>MGGEIITLQAGQCGNHVGKFLWSQLAKEHAIGTDGLSQLPDSSTERDDDTKPFFRENSRNKFTPRAIMMDSEPSVIADVENTFRGFFDPRNTWVASDGASAGNSWANGYDIGTRNQDDILNKIDKEIDSTDNFEGFQLLHSVAGGTGSGLGSNLLEALCDRYPKKILTTYSVFPARSSEVVVQSYNTILALRRLIEDSDATVVFDNASLLNISGKVFRNPNIDLQHTNQLISTIISSVTNSIRFPSYMYSSMSSIYSTLIPSPELHFLSPSFTPFTSDYIHDDIAHKGHSSYDVMLDLLDPSNSLVSTAMNNPTYFNVYNTIIGNVEPRQISRAMTKLQQRIKFPSWSSSAMHVNIGRRSPYLPLQPNENEVSGMMLSNMSTVVNVFENACNTFDKVFAKGAFLNNYNVGDLFQSMQNVQDEFAESREVVQSLMEDYVAAEQDSYLDDVLVDDENMVGELEEDLDADGDHKLV[2x];> MEIKEVDDRAELLRYTNNIPLLGKLVNHQPLWSTNPKLKSFSLEKISAPDQRRVQEALVVKDLLNVLIGLEGTYIRYFNDYEPSDPETPIEFKIAKKMDPSFKTFSRRIVRYGKQYMILTRAYEKWSDTSFGMVLQRFAYEIRRFLEDVYLKTLVERLERDFNKVPNFSIRELEQIINETEVNKQMELLYNIYEEIFREIEERRTNQSSQEDFNNFMDSMKNESSLHLRLMVAFDTTVYPVPKGGAILKIFQQKILENLGDRSSVMFLKKLLNNISQDYCTMLYEWLTQGILNDPYQEFMTYDDLEGKTDNIFDTRDRAWDTQYFIRKDVLLRDCDSEEDKNLLFKMLRTGILLKVVRASLQIPTIPSNSSDITIQEINDFADLMEGSNLELYVDKCYSRANEIFLKLFFQGYDLINVLKHLQQIFLGYQSGHNVLKFLTKNMGELTKHYRNDNNANYDKLLQNFELERQSENPNNLMRQLLMIQFDTETLPQVLSHYLQIYPEVPENNSANDDSDPLMHANNFKNMNAILFDELSKERTGAYHGSNLELYTPKSAIYHLKFDINIPYPLNIIISRTCMIKYQIILRYQLVLQYHSRLLDETWMDLNKTPSWKYRGYSHTVKRRIVRATRVLHAKMNHFIKTIMEYFNQNVIDKEVYSLEKCYRNPTLAVAIQNELEGGLTNIMTNRCLSDLIPLQLQIFDIVYKFCKFIKSMRAKLCQLDPVLYEKHKSGMMKTLNEGYRTNNGGQEDVGYQEDAALELIQKLIEYISNASSIFRKCLINFTQELSTEKFDFYDSSSVDAAGIERVLYSIVPPRSASASSQR;> MELEPTLFGIIEALAPQLLSQSHLQTFVSDVVNLLRSSTKSATQLGPLIDFYKLQSLDSPETTIMWHKIEKFLDALFGIQNTDDMVKYLSVFQSLLPSNYRAKIVQKSSGLNMENLANHEHLLSPVRAPSIYTEASFENMDRFSERRSMVSSPNRYVPSSTYSSVTLRQLSNPYYVNTIPEEDILKYVSYTLLATTSALFPFDHEQIQIPSKIPNFESGLLHLIFEAGLLYQSLGYKVEKFRMLNISPMKKALIIEISEELQNYTAFVNNLVSSGTVVSLKSLYREIYENIIRLRIYCRFTEHLEELSGDTFLIELNIFKSHGDLTIRKIATNLFNSMISLYYEYLMNWLTKGLLRATYGEFFIAENTDTNGTDDDFIYHIPIEFNQERVPAFIPKELAYKIFMIGKSYIFLEKYCKEVQWTNEFSKKYHVLYQSNSYRGISTNFFEIINDQYSEIVNHTNQILNQKFHYRDVVFALKNILLMGKSDFMDALIEKANDILATPSDSLPNYKLTRVLQEAVQLSSLRHLMNSPRNSSVINGLDARVLDLGHGSVGWDVFTLDYILYPPLSLVLNVNRPFGRKEYLRIFNFLWRFKKNNYFYQKEMLKSNDIIRSFKKIRGYNPLIRDIINKLSRISILRTQFQQFNSKMESYYLNCIIEENFKEMTRKLQRTENKSQNQFDLIRLNNGTIELNGILTPKAEVLTKSSSSKPQKHAIEKTLNIDELESVHNTFLTNILSHKLFATNTSEISVGDYSGQPYPTSLVLLLNSVYEFVKVYCNLNDIGYEIFIKMNLNDHEASNGLLGKFNTNLKEIVSQYKNFKDRLYIFRADLKNDGDEELFLLSKSLR;> MDEASHLPNGSLKNMEFTPVGFIKSKRNTTQTQVVSPTKVPNANNGDENEGPVKKRQRRSIDDTIDSTRLFSEASQFDDSFPEIKANIPPSPRSGNVDKSRKRNLIDDLKKDVPMSQPLKEQEVREHQMKKERFDRALESKLLGKRHITYANSDISNKELYINEIKSLKHEIKELRKEKNDTLNNYDTLEEETDDLKNRLQALEKELDAKNKIVNSRKVD

Microtubule (MT) nucleation is regulated by the γ-tubulin ring complex (γTuRC), conserved from yeast to humans. In budding yeast, homologues of the grip-containing proteins (GCPs) GCP2 and GCP3 (Spc97p and Spc98p) and two copies of γ–tubulin (Tub4p) form a 300 kDa complex (γTuSC). Spc110p, a distant pericentrin homologue, recruits this complex to the nuclear face of the spindle pole body (SPB), while Spc72p recruits it to the cytoplasmic face. In yeast, the CM1 motif is required for seven identical γTuSCs to helically assemble into a γTuRC at the SPB.

Previous moderate-resolution cryo-EM structural studies (8 Å) had shown that wild-type (WT) yeast γTuSCs complexed with the N-terminal domain of Spc110p self-assemble into helical filaments (hereafter γTuRC) having 6.5 γTuSCs/turn, thereby presenting 13 γ-tubulins to template 13-protofilament MTs. Although close to MT symmetry, the γ-tubulins within each γTuSC were too far apart to correctly match the MT lattice, adopting an open conformation. Realizing that this would require much higher resolution of Spc110p-γTuSC interactions, we focused on obtaining higher resolution structures of the ‘open’ (γTuRCWT) and disulfide trapped ‘closed’ (γTuRCSS) filaments containing Spc110p by collecting new datasets on a direct electron detector and incorporating symmetry expansion and 3D classification into the data processing pipeline. To improve the resolution, we performed symmetry expansion followed by focused classification of segments containing three adjacent γTuSCs. The resulting reconstructions were at a resolution of 3.6 Å and 3.0 Å for the γTuRCWT and γTuRCSS filaments, respectively (Figure 3—figure supplements 1–3). During the transition from monomer to assembled open state (as seen in γTuRCWT), the γ-tubulins move in the same overall direction, approximately orthogonal to the plane of the Spc97p/Spc98p contact interface. The center of mass of the γ-tubulins shifts ~13.8 Å and ~15.6 Å when bound to Spc97p and Spc98p, respectively, as a result of twisting the helical bundles in Spc97p and Spc98p. Notably, much of the bottom three helical bundles show only minor changes when assembling to the open state. The dominant changes occur on loop Spc98pH10-S1 in the middle contact, which moves ~4.1 Å, and at the N-terminus of helix Spc98pH11, involved in the top contact, which moves ~6.6 Å. During the transition from the assembled open γTuRCWT to the engineered γTuRCSS closed conformation, the γ-tubulins on Spc97p and Spc98p slide past each other in roughly opposite directions, undergoing translations of ~6.9 Å and ~7.7 Å, respectively. Overall, these conformational changes alter the pitch and twist of the γTuRC assemblies from ~140 Å/turn and 54.5o in the open state to ~132 Å/turn and 55.1o in the closed state.> MLFYSFFKTLIDTEVTVELKNDMSIRGILKSVDQFLNVKLE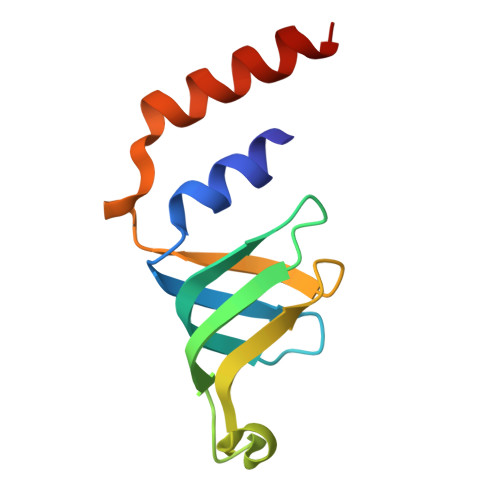NISVVDASKYPHMAAVKDLFIRGSVVRYVHMSSAYVDTILLADACRRDLANNKRQ> MAHFPDTPAFTGFNAPSRIECDIPNLVHEGTIPPELNGAFFRVQPDPQFPPRLGDDISFNGDGMITRFHIHDGQCDIKQRWAKTNKWKLENAAGKALFGSYRNPLTDDESVKGEYRSTANTNAFVFAGKLWAMKEDSPSLTMDPATMETFGFEKFGGKMTGQTFTAHPKVDPLTGNMVAIGYAASGLCTDDVCLYEISPDGELIYEAWFKVPYYCMMHDFGVTKDYLVLHIVPSIGSWDRLEKGLPHFGFDTTLPVYLGIIPRRADLKQEDIRWFKRENCFASHVMNAFQEGTKVHVDVPEAENNMFPFFPDVHGAPFNPQQAMSRLTRWTVDMASNSDEFDSVTRLTETAGEFPRIDDRMTGLPYRYGWMLEMDMKRPVELKGGSAGGFLMNCLFLKDHQTGAEQHWWCGPTSSLQEPAFIPRSKDAPEGDGWIVQVCNRLADHKSDLLIFEALDIEKGPVATVHLPFALRFGLHGNWANAEEIGLAA

Lignostilbene-α,β-dioxygenases (LSDs) are iron-dependent oxygenases involved in the catabolism of lignin-derived stilbenes. LSDs are nonheme iron enzymes that catalyze the O2-dependent cleavage of trans-4-hydroxystilbenes to yield two aromatic aldehydes. LSD4 catalyzed the cleavage of DCA-S to 5-formylferulate and vanillin and cleaved lignostilbene and DCA-S (∼106 M−1 s−1) with tenfold greater specificity than pterostilbene and resveratrol. The overall structure of LSD4 is typical of CCDs: a seven-bladed β-propeller fold with a cap-like feature on one face formed by extended loops.

To facilitate the structural characterization of LSD4·substrate complexes, we generated Co-LSD4 in which the catalytic Fe2+ was substituted with Co2+. This metal ion substitution in CAO1 yielded an inactive but isostructural enzyme. Co-LSD4 was produced by growing cells producing LSD4 in a minimal medium supplemented with Ca2+, Mg2+, and Co2+ as the only divalent metal ions. Inductively coupled plasma–mass spectrometry (ICP-MS) analysis revealed that each protomer of Co-LSD4 contained 0.92 ± 0.06 equivalents of Co2+ and ∼0.02 equivalents of Fe2+. Co-LSD4 had a faint purple hue and a λmax of ∼480 nm. Finally, incubating lignostilbene with Co-LSD4 led to rates of O2 consumption that were barely above background. This is consistent with Co-LSD4 being inactive, with residual activity in the preparation the result of trace Fe-LSD4. Therefore, we prepared catalytically inactive Co-LSD4, a strategy that yielded ligand-bound structures of CAO1 (31, 32). Co-LSD4 crystallized under similar conditions as native enzyme and the two structures were nearly identical, with an RMSD of 0.1 Å over 471 aligned Cα atoms. The coordination geometry of the active site metal ion was also highly similar in the two variants.>[2x]MAYRIVSETGDKITVELTLANKNTHYVWNGWCFDIKNITFETTGKVLSIKYADGGEPVYNVNGNLVTIDLTWRGIFHLNTTVKIIIEIQKSGDNPYPHNFKIHYLRGESIIYPTIGELPASWKPGNFTLSDLIADPKSYYDPHVKPHQNGFIMY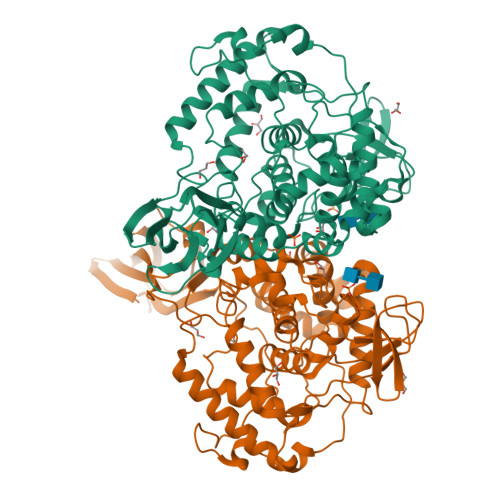NPPHPTQIIIGLADIDYPLNLASSARMWVPNKYFAMGLALAYEWFKVNPNFLMALAAKENWGTAVTKDPAFKGYKVIIDEEEYYWPVQIDHPDGIFQVESGNFNQIKAYYPDIFPDTADHDDYMKVSLDPNDTAWITSPIVAAVSLTMERELLYAAVGDKYNEFLRLAKDPWAETEIIDFGYNRGVGAIEALKIFSDNWEKAINAEVLWKEFNMEGFGGHVPTVINITATMDMETERIYDANLTWDDIEYFFTVVRQKFFRPGAISDEEWNAMMRDVKRAYDLLSQHWGGDHISYRYDFLTILRVAMKHWPEPHIPRPTGDDWYYHARNYNP> ATSDSNMLLNYVPVYVMLPLGVVNVDNVFEDPDGLKEQLLQLRAAGVDGVMVDVWWGIIELKGPKQYDWRAYRSLLQLVQECGLTLQAIMSFHQCGGNVGDIVNIPIPQWVLDIGESNHDIFYTNRSGTRNKEYLTVGVDNEPIFHGRTAIEIYSDYMKSFRENMSDFLESGLIIDIEVGLGPAGELRYPSYPQSQGWEFPGIGEFQCYDKYLKADFKAAVARAGHPEWELPDDAGKYNDVPESTG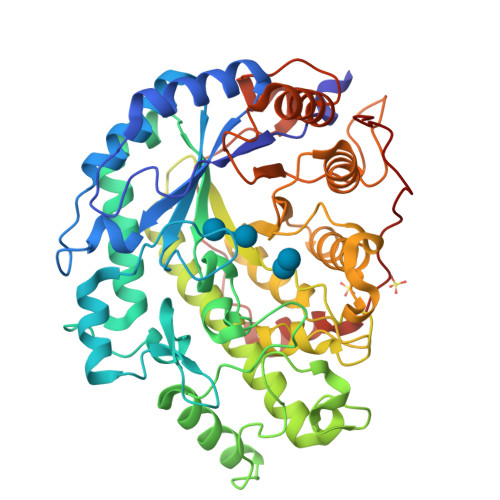FFKSNGTYVTEKGKFFLTWYSNKLLNHGDQILDEANKAFLGCKVKLAIKVSGIHWWYKVENHAAELTAGYYNLNDRDGYRPIARMLSRHHAILTFTCLEMRDSEQPSDAKSGPQELVQQVLSGGWREDIRVAGENALPRYDATAYNQIILNARPQGVNNNGPPKLSMFGVTYLRLSDDLLQKSNFNIFKKFVLKMHADQDYCANPQKYNHAITPLKPSAPKIPIEVLLEATKPTLPFPWLPETDMKVDG>MVPTRSTARMLANLKIRTGMFWVLSLFSLTLLFSTASAWWAALGSDQQITELDQTAHQSDRLNNALLMAIRSSANVSSGFIEQLGGHDESAGKRMALSVELNNKSQALVDEFVENAREPALRGLATELQATFAEYAKAVAGQREATRQRSLEQYFKVNSDAGNAMGRLQTLRQQLVTTLSERGQQIMLESDRRLARAQLLSLCLLGVTVVLAVLCWAFIAQRVLHPLREAGGHFRRIASGDLSVPVQGQGNNEIGQLFHELQRMQQSQRDTLGQINNCARQLDAAATALNAVTEESANNLRQQGQELEQAATAVTEMTTAVEEVARNAITTSQTTSESNQLAAQSRRQVSENIDGTEAMTREIQTSSAHLQQLVGQVRDIGKVLEVIRSVSEQTNLLALNAAIEAARAGE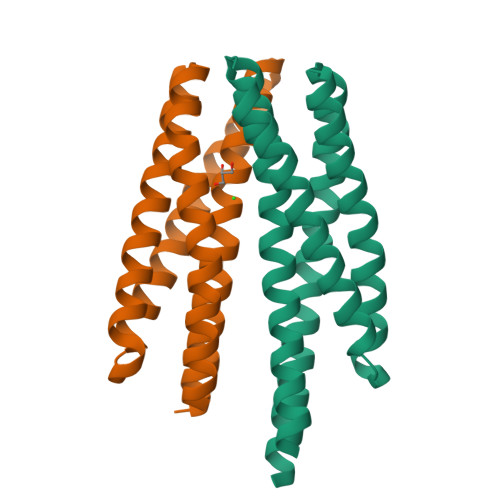AGRGFAVVADEVRTLAYRTQQSTQEIEQMIGSVQAGTEAAVASMQASTNRAQSTLDVTLASGQVLEGIYSAIGEINERNLVIASAAEEQAQVAREVDRNLLNIRELSNHSAAGAQQTSEASKALSGLVGEMTALVGRFKV[2x]> MRGSAHVVILGAGTGGMPAAYEMKEALGSGHEVTLISANDYFQFVPSN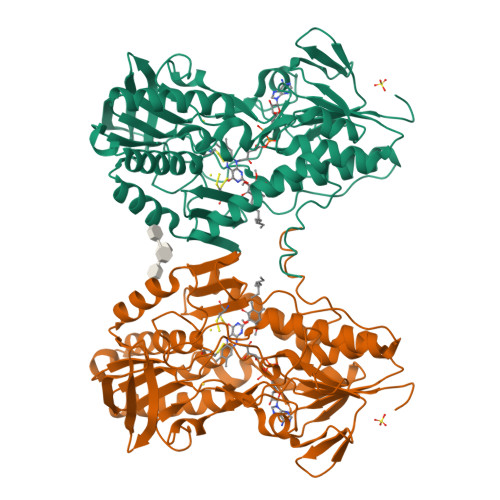PWVGVGWKERDDIAFPIRHYVERKGIHFIAQSAEQIDAEAQNITLADGNTVHYDYLMIATGPKLAFENVPGSDPHEGPVQSISTVDHAERAFAEYQALLREPGPIVIGAMAGASCFGPAYEYAMIVASDLKKRGMRDKIPSFTFITSEPYIGHLGIQGVGDSKGILTKGLKEEGIEAYTNCKVTKVEDNKMYVTQVDEKGETIKEMVLPVKFGMMIPAFKGVPAVAGVEGLCNPGGFVLVDEHQRSKKYANIFAAGIAIAIPPVETTPVPTGAPKTGYMIESMVSAAVHNIKADLEGRKGEQTMGTWNAVCFADMGDRGAAFIALPQLKPRKVDVFAYGRWVHLAKVAFEKYFIRKMKMGVSEPFYEKVLFKMMGITRLKEEDTHRKAS> GGCUUCAACAACCCCGUAGGUUGGGCCGAAAGGCAGCGAAUCUACUGGAGCC

The nadA motif is the first known NAD+-dependent riboswitch, comprising two similar tandem bulged stem–loop structures. A 52 nt RNA with the sequence of the Candidatus koribacter versatilis NAD+ riboswitch domain 1 was made by chemical synthesis and cocrystallized with a number of ligands related to NAD+. We find that helices P1, P1a, and P1b are coaxial, with a base paired interaction between the ACANCCCC bulge and the internal loop generating a pseudo-three-way junction that creates a binding site for ADP and related compounds. The adenine nucleoside of the ligand is hydrogen bonded to the riboswitch RNA, and the phosphate groups interact directly with one of two magnesium ions bound in the narrow neck of the ACANCCCC bulge.

However, using in-line probing Malkowski et al. (2019) measured binding isotherms that provided no evidence for cooperative binding. Their probing experiments also indicated that only the ADP moiety of NADH (and ADP itself as well as a number of derivatives including AMP and ATP) bound to domain 1. Malkowski et al. (2019) showed that a number of ADP derivatives bound to domain 1, and this provides the means to explore the generality of ligand binding by this RNA. For each ligand the structure of the RNA is essentially unaltered with an average overall RMSD of 0.27 Å, and the manner of ligand binding is also closely similar. The binding of the adenosine moiety is essentially the same for each compound, with the adenine nucleobase stacked with A8 and its N1, N3, and O2′ hydrogen bonded to the RNA in an identical manner. The phosphate groups all make very similar interactions with the M2 metal ion, in most cases nonbridging oxygen atoms of both α and β phosphates bonding directly to the metal atom. 5-Bromocytosine was incorporated at position 3 or positions 42 and 45 in the P1 helix in order to provide phase information. These species crystallized in space group I222, with good resolution, and some of the structures were solved using SAD from the bromine atoms.>DSIIHIGAIFDESAKKDDEVFRTAVGDLNQNEEILQTEKITFSVTFVDGNNPFQAVQEACELMNQGILALVSSIGCTSAGSLQSLADAMHIPHLFIQRS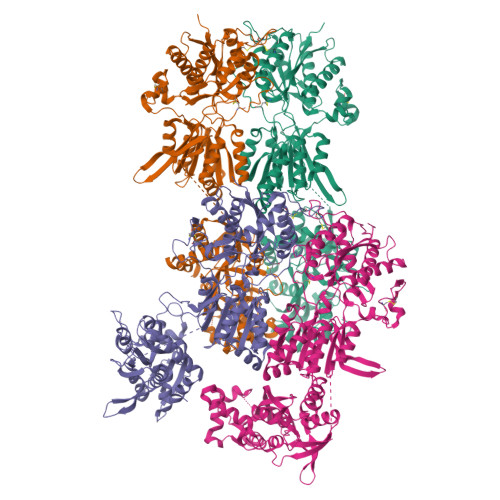TAGTPRSGCGLTRSNRNDDYTLSVRPPVYLNEVILRVVTEYAWQKFIIFYDSEYDIRGIQEFLDKVSQQGMDVALQKVENNINKMITTLFDTMRIEELNRYRDTLRRAILVMNPATAKSFISEVVETNLVAFDCHWIIINEEINDVDVQELVRRSIGRLTIIRQTFPVPQNISQRCFRGNHRISSTLCDPKDPFAQNMEISNLYIYDTVLLLANAFHKKLQDRKWHSMASLSCIRKNSKPWQGGRSMLETIKKGGVNGLTGDLEFGENGGNPNVHFEILGTNYGEELGRGVRKLGCWNPVTGLNGSLTDKKLENNMRGVVLRVVTVLEEPFVMVSENVLGKPKKYQGFSIDVLDALSNYLGFNYEIYVAPDHKYGSPQEDGTWNGLVGELVFKRADIGISALTITPDRENVVDFTTRYMDYSVGVLLRRAEKTVDMFACLAPFDLSLWACIAGTVLLVGLLVYLLNWLNPPRLQMGSMTSTTLYNSMWFVYGSFVQQGGEVPYTTLATRMMMGAWWLFALIVISSYTANLAAFLTITRIESSIQSLQDLSKQTDIPYGTVLDSAVYQHVRMKGLNPFERDSMYSQMWRMINRSNGSENNVLESQAGIQKVKYGNYAFVWDAAVLEYVAINDPDCSFYTVGNTVADRGYGIALQHGSPYRDVFSQRILELQQSGDMDILKHKWWPKNGQCDLYSSVDAKQKGGALDIKSLAGVFCILAAGIVLSCLIAVLETWWSRRKGSRVPSKEDDKEIDLEHLHRRVNSLCTDDDSPHKGLVPRGS[4x]> SPSPSP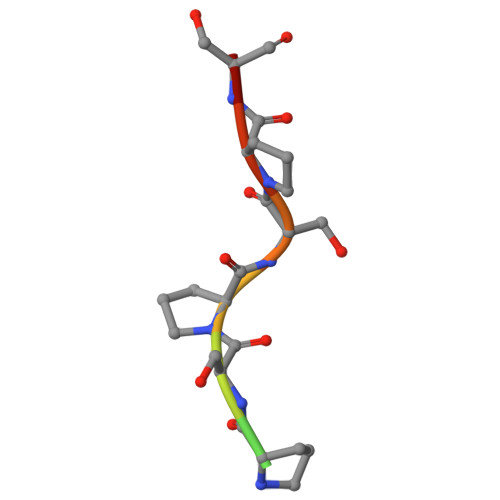SPSP>MDKFRVQGPTRLQGEVTISGAKNAALPILFAALLAEEPVEIQN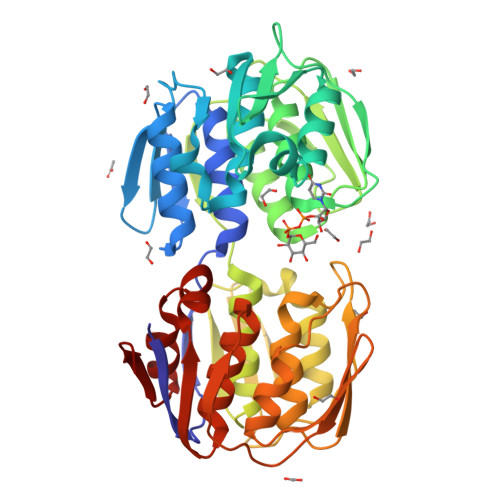VPKLKDIDTTMKLLTQLGTKVERDGSVWIDASNVNNFSAPYDLVKTMRASIWALGPLVARFGQGQVSLPGGCAIGARPVDLHIFGLEKLGAEIKLEEGYVKASVNGRLKGAHIVMDKVSVGATVTIMSAATLAEGTTIIENAAREPEIVDTANFLVALGAKISGQGTDRITIEGVERLGGGVYRVLPDRIETGTFLVAAAISGGKIVCRNAQPDTLDAVLAKLREAGADIETGEDWISLDMHGKRPKAVTVRTAPHPAFPTDMQAQFTLLNLVAEGTGVITETIFENRFMHVPELIRMGAHAEIESNTVICHGVEKLSGAQVMATDLRASASLVLAGCIAEGTTVVDRIYHIDRGYERIEDKLRALGANIERVKGE[4x]>MTKWVLHVDLDQFYASVELRRRPDLRGQPVIVGGSGDPSEPRKVVTCASYEAREFGVHAGMPLRAAARRCPDATFLPSDPAAYDEASEQVMGLLRDLGHPLEVWGWDEAYLGADLPDESDPVEVAERIRTV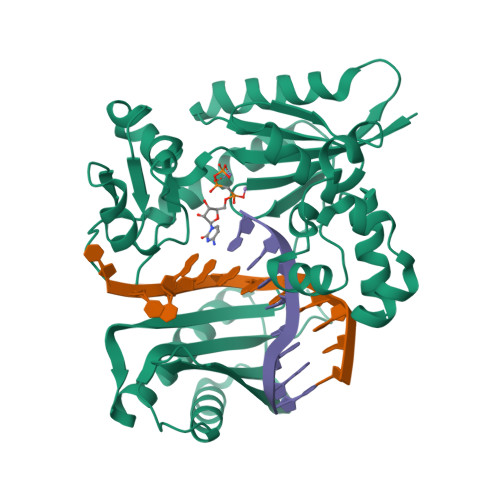VAAETGLSCSVGISDNKQRAKVATGFAKPAGIYVLTEANWMTVMGDRPPDALWGVGPKTTKKLAAMGITTVADLAVTDPSVLTTAFGPSTGLWLLLLAKGGGDTEVSSEPWVPRSRSHVVTFPQDLTERREMDSAVRDLALQTLAEIVEQGRIVTRVAVTVRTSTFYTRTKIRKLPAPSTDAGQIVDTALAVLDQFELDRPVRLLGVRLELAMDDVPRPAVTAGT[2x]>[2x]MVIGRVVNEMEVGVPADDIWAVYSSPELPRLFVQLMPNVYKKIDILQGDGTVGTVLHIELADGIPEPRTWKEKFIKIDHQHREKVVRQIEGGFLDMGFRVFDVIFKIIEKD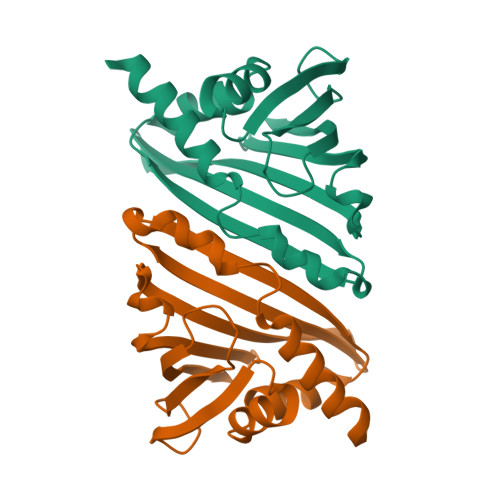ACSCIIRSTTAFELDEKFENNANLITAGNLWGAAKAISNYVIQNKSKRRNH>[4x]MVKVDLESKRYGEKLKEVFLMLDNNVVECIKEITESSRNGKLVFFVGAGVSTLSDYPQWWRLVDKYHEELYGSPKKGNYSSDEYLRIPQIFYNVKGEMAFDGILKDFFQVDKPTNPIHDKILAMNPAHVITTNYDNLIDTACWKRGKYFSVISAEEDVANATSSRYLLKVHGDFRKGFKGENVVLKEDDYLNYDQNYPLISNLMKTIIATHTIVFIGYGLGDYNINMLLNWVRKLQKDSFHKPFFIRTDPSPIENETLIYYENKGLRIIDAASLIDSNEYDYLERYSAVMDLLIESQENKFITKDDEVIDYIYGKISPLFALQYIRKIDLKHVFEYDYHFEVNGTVVRHKNKGFGYMERFFELKESC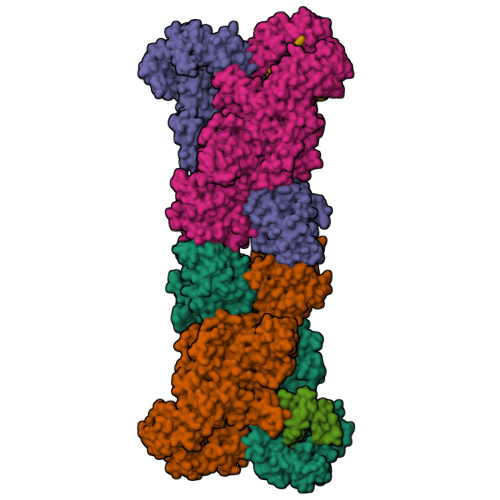DERSKLSKKQYERFNALFNFFEKNGVICMAKDAGTLNTSIEINSLAYHGKYDVMKKFIEEQSVSIEDDYKKAFFLACLGRWEESYDLYSNIILNSIDESNGCVYYLSQINRYRIYQSITQAVTQFNGLGLLTFGRHYKPFTDEFLARIEREMTNFNIDDLFNGMPFEFQKKYKILEFLSDNQFLYDDTVKLFELTNKVRSEMSEGSYSFGMSSDIVVLLRLYDNLRFLYENCLWSVSFHEFHQYIRNSMSLLIEKAEYERTRDIDELGFSFFGKKSGFFMEYYDFVNISRHFKIDDIKNLERSCSIDKIRFGEQEKIEEYLVGIAEEITKQFSANGMNVVFYTQFISEAKAALYFAKYVKLSEEGLGKIVKALLFYFPERDLDIGKRYVWLERLTKCNELPKSIISIIDDFLVLQAEKHIDQNYSEVSSNGLYSRDYGALIKHFEKNFISKRLSEITLCLTQDKQKQIDFLFKLLPLLSTNAKSHLLSFKSVENINDLMNGIRIGLIDEFTPEHEELIIEYLETRKVNYIVEKEKGIQTFSSNDYMSTFGIWYFLEEINNSKMEEFIGMDDQYDFFVDPENFDYKKFIPSWLKNYNDKLLGKIAGNKHMKHHVIEVLKERVKNSNDKRYLEILMNYFI;>[2x]MIEIFKDTGATHDLVYHSKINTFVWDVEFDIVLSDSKELNKCYFVKCFNPYRINGKCDFAVSSIDIFSEGKRLLIENEFNFKITKAVHVATSKDVTEIVLHLSERISSPFPIVKEVVYLD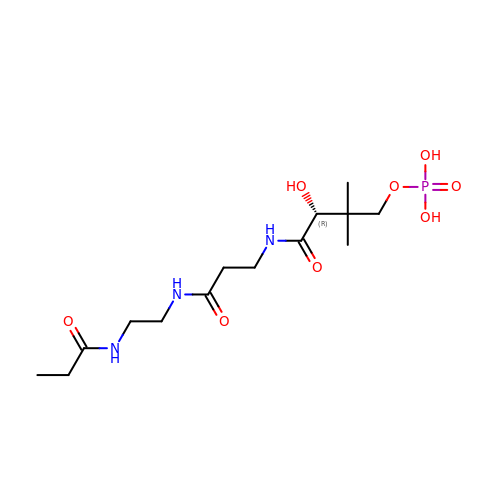N~3~-[(2R)-2-hydroxy-3,3-dimethyl-4-(phosphonooxy)butanoyl]-N-[2-(propanoylamino)ethyl]-beta-alaninamide | C14 H28 N3 O8 P | IEZRALNUCGHOKF-LBPRGKRZSA-N>[2x]GMENEENSAREQEADDFLHIASVKEDWGGDGRGRMNLSGRRTAIAKEYLPRQYQFFDTNTVMEKQGWRVRGMPDNIAPGSRRLLTWHDSGASTSRVVLPPKFEAPSGIFTADLEIFVIKGAIQLGEWQL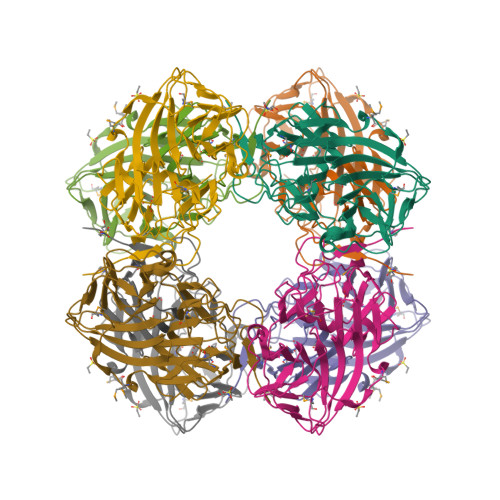NKHSYSFIPAGVRIGSWKVLGGEEAEILWMENGSVPLEYKYAQEDHPDARLSDFIPALDSKLLPWGKADTVQFVQANKKWLRKDINGGGVWLLAILPHFDNKYQMIQPYNEEGYCLTGYCDVGDYRIVKDHYWYCPSFSTLPRHITDDGGLFFVRVDRDLSKVATVLSYAPQDT methyl N-(2-{[(2M)-2-(pyridin-3-yl)-1,3-thiazole-4-carbonyl]amino}prop-2-enoyl)-D-alaninate | 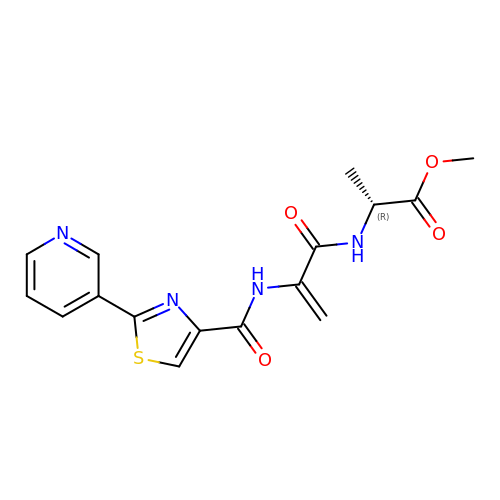C16 H16 N4 O4 S | RVPKOYWAKLWTTB-SNVBAGLBSA-N>[2x]MKETILVNL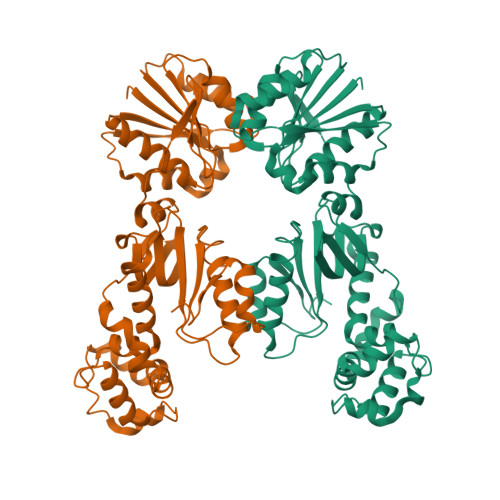VSEQTIPNVQFIKWYFNKKQTPMKILLVSTKEMEQKEKSLFIKNALHFSDSFVEWETIHTDGNDISKTENILTDYFRDNEYKNIIVNITGGTKIMSLAAFDFFNNKPNTEIFYQPIGKELQELYPNKQKYDMFEVLSLKEYLDAHGISYKYDNECVKDWNYNKTVYDLCVADNRELIKGMIALQNNSYFNNVYKRKDFLDFTQIEEEKFIAINHPAATKENMIKILQIFGFDVSRIEHKHIRYITGGWFEEYVYQKICNEYHNVDEKNVALNVTIQKGNDKNELDVIYLDKDNKLHVIECKSFVDGNEGNRVLNDALYKLQAIIKSKFGLYVKQHLYTKSIIEKETPLNRAKEFGIDIKDGTQLGSGHHHHHH> VPPGGEPLYTEQDLAVNGREGFPNYRIPALTVTPDGDLLASYDGRPTGIDAPGPNSILQRRSTDGGRTWGEQQVVSAGQTTAPIKGFSDPSYLVDRETGTIFNFHVYSQRQGFAGSRPGTDPADPNVLHANVATSTDGGLTWSHRTITADITPDPGWRSRFAASGEGIQLRYGPHAGRLIQQYTIINAAGAFQAVSVYSDDHGRTWRAGEAVGVGMDENKTVELSDGRVLLNSRDSARSGYRKVAVSTDGGHSYGPVTIDR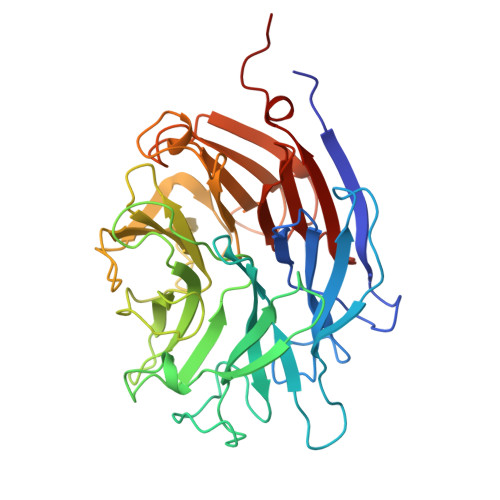DLPDPTNNASIIRAFPDAPAGSARAKVLLFSNAASQTSRSQGTIRMSCDDGQTWPVSKVFQPGSMSYSTLTALPDGTYGLLYEPGTGIRYANFNLAWLGGICAP> DRSLRAVPGGSSPAWTQCQQLSQKLCTLAWSAHPLVGHMDLREEGDEETTNDVPHIQCGDGCDPQGLRDNSQFCLQRIHQGLIFYEKLLGSDIFTGEPSLLPDSPVGQLHASLLGLSQLLQPEGHHWETQQIPSLSPSQPWQRLLLRFKILRSLQAFVAVAARVFAHGAATLSPHHHHHH;> DRSLIWELKKDVYVVELDWYPDAPGEMVVLTCDTPEEDGITWTLDQSSEVLGSGKTLTIQVKEFGDAGQYTCHKGGEVLSHSLLLLHKKEDGIWSTDILKDQKEPKNKTFLRCEAKNYSGRFTCWWLTTISTDLTFSVKSSRGSSDPQGVTCGAATLSAERVRGDNKEYEYSVECQEDSACPAAEESLPIEVMVDAVHKLKYENYTSSFFIRDIIKPDPPKNLQLKPLKNSRQVEVSWEYPDTWSTPHSYFSLTFCVQVQGKSKREKKDRVFTDKTSATVICRKNASISVRAQDRYYSSSWSEWASVPCSHHHHHH;> DTLTKSFCYFGTWCQMYGST

IL-23 is a heterodimeric cytokine comprised of p19 and p40 subunits and plays a key role in establishing autoimmune diseases such as psoriasis, arthritis, inflammatory bowel disease, and colitis. IL-23 and IL-12 share a common subunit, p40, therefore library selection against IL-12 should remove the p40 binders. IL-23R interacted strongly to wild-type and most of ala-mutants, except for clones with alanine mutation at residues 137, 141, and 145 of p19. These residues, in particular W137, have previously shown to be major sites for receptor binding.

Sequence analysis of specific p19 binders indicated that more than 40% of clones share a common motif comprised of phenylalanine-Glycine-Leucine/Threonine (FGL/T). Binding of two FGL containing peptides on-phage, 23–644 and 23–652 to IL-23 was confirmed in a titer dependent phage ELISA. Fab-phage bound strongly to wild-type IL-23 and not to W137 and K145 ala-mutants of p19. Both FGL-phage bound to wild-type IL-23 and its ala-variants including Ala137, except for Ala26. HDX-MS results for peptide 23–652 showed decreased deuterium uptake in Helix A at amino acids 15–33 (QQLSQKLCTLAWSAHPLVG) and decreased deuterium exchange in the D1 region of the p40 subunit at amino acids 293–299 (YSSSWSE). A crystal structure of IL-23 in complex with 23–652 was determined and confirmed the HDX result. The co-crystal structure revealed that all interactions of the peptide 23–652 with IL-23 are confined to p19 helix A, a small section of the p19 AB loop, and D3 of p40. In particular Trp26 (p19) was flipped out relative to the apo structures to pick up an interaction with Phe7 of 23–652. HDX and co-crystal structure results confirmed the earlier finding that W26 is in fact a hotspot residue for binding of peptides 23–644 and 23–652, since neither one of the peptides retained binding to the W26A mutant of IL-23. As expected FGLT-containing peptide, 23–652 was confirmed as non-blocker.> GPAVPRMDTTIDGFADSYEISSTSFVATDNTDSSIVYLAAEQVLTGPDVSALQLLSNSFESVFDSPDDFYSDAKLVLSDGREVSFHRCVLSARSSFFKSALAAAKKEKDSNNTAAVKLELKEIAKDYEVGFDSVVTVLAYVYSSRVRPPPKGVSECADENCCHVACRPAVDFMLEVLYLAFIFKIPELITLYQRHLLDVVDKVVIEDTLVILKLANICGKACMKLLDRCKEIIVKSNVDMVSLEKSLPEELVKEIIDRRKELGLEVPKVKKHVSNVHKALDSDDIELVKLLLKEDHTNLDDACALHFAVAYCNVKTATDLLKLDLADVNHRNPRGYTVLHVAAMRKEPQLILSLLEKGASASEATLEGRTALMIAKQATMAVECNNIPEQCKHSLKGRLCVEILEQEDKREQIPRDVPPSFAVAADELKMTLLDLENRVALAQRLFPTEAQAAMEIAEMKGTCEFI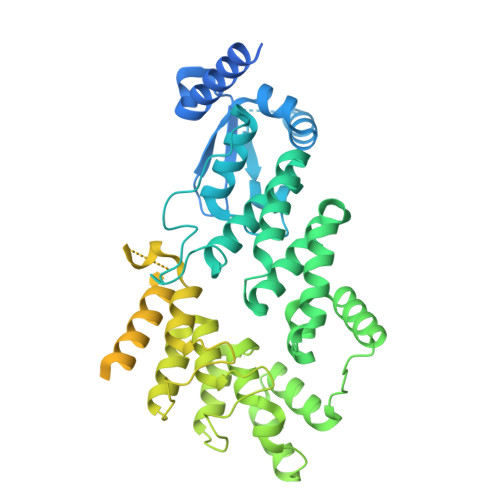VTSLEPDRLTGTKRTSPGVKIAPFRILEEHQSRLKALSKTVELGKRFFPRCSAVLDQIMNCEDLTQLACGEDDTAEKRLQKKQRYMEIQETLKKAFSEDNLELGNSSLTDSTSSTSKSTGGKRSNRKLSHRRRGGWSHPQFER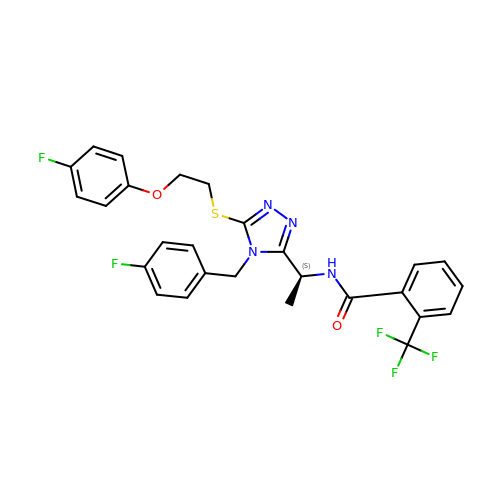N-[1-(5-{[2-(4-fluorophenoxy)ethyl]sulfanyl}-4-[(4-fluorophenyl)methyl]-4H-1,2,4-triazol-3-yl)ethyl]-2-(trifluoromethyl)benzamide | C27 H23 F5 N4 O2 S | SZVUNXFRJYHQBI-KRWDZBQOSA-N> GPGSMNSPPKVSVLITVTGVDQPGVTATLFEVLSRHGVELLNVEQVVIRHRLTLGVLVCCPADVADGPALRHDVEAAIRKVGLDVSIERSDDVP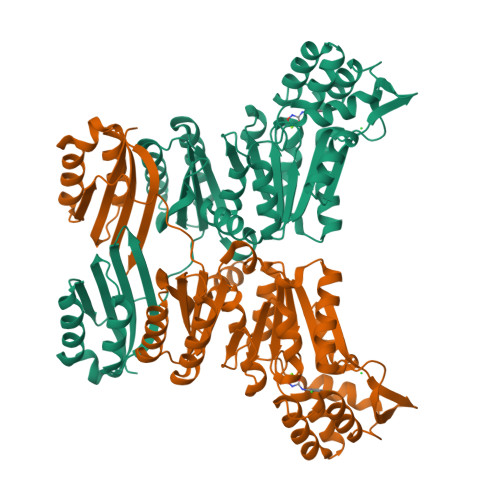IIREPSTHTIFVLGRPITAAAFGAVAREVAALGVNIDLIRGVSDYPVIGLELRVSVPPGADEALRTALNRVSSEEHVDVAVEDYTLERRAKRLIVFDVDSTLVQGEVIEMLAAKAGAEGQVAAITDAAMRGELDFAQSLQQRVATLAGLPATVIDEVAGQLELMPGARTTLRTLRRLGYACGVVSGGFRRIIEPLAEELMLDYVAANELEIVDGTLTGRVVGPIIDRAGKATALREFAQRAGVPMAQTVAVGDGANDIDMLAAAGLGIAFNAKPALREVADASLSHPYLDTVLFLLGVTRGEIEAADAIDGEVRRVEIPPE> SGRAWDGLWDPTLPMIPSANIPGDPI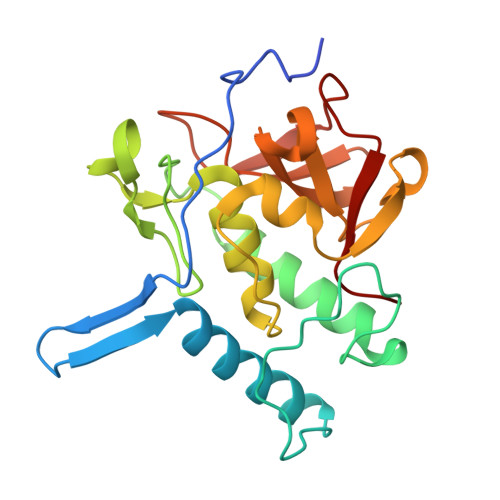AVVNQVLGISATSAQVTANMGRKFLEQLGILQPTDTGITNAPAGSAQGRIPRVYGRQASEYVIRRGMSQIGVPYSWGGGNAAGPSKGIDSGAGTVGFDCSGLVLYSFAGVGIKLPHYSGSQYNLGRKIPSSQMRRGDVIFYGPNGSQHVTIYLGNGQMLEAPDVGLKVRVAPVRTAGMTPYVVRYIEY>[12x]GSHMGTVRQTSGPALARGD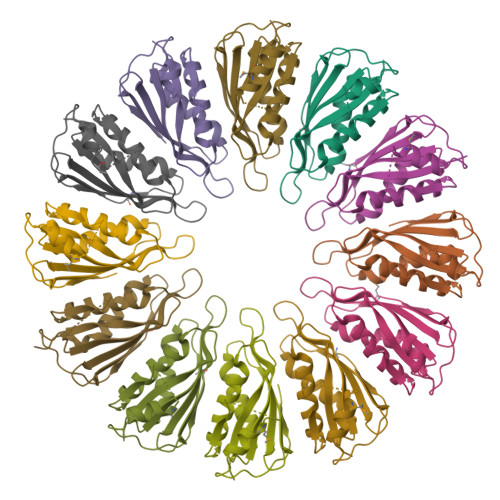KVAVVSIANYTETPDAGHSAESIAANTLRAGGIADVRIAPADSNRNSLFDTTQRADSDKAMEWARSQNARYVLSGAVEEWRYKTGVDGEPVVGVTFELIDVSNGAVVWSATGTRTGWSRSGLSSVATSLIAKVLSPLQARQ>MSGSPAPQGALRQRIVASTPKKTKESKDGAASDAELDKLVKEAAAAKAPAGSERDYKIAFAIITALAFLTRFWGISHPDQVVFDEVHFGKFASYYLQRTYFFDVHPPLGKLLFAFMGWLVGYDGHFHFDNIGDPYVINKVPYVAFRALPAILGSLTVSVVFLIMWESGYSLPACILASGLVLLDNAHIGQTRLILLDATLVFAMACSLLCYIKFYKLRHEPFSRKWWKWLILTGFALSCDISTKYVGLFAFITIGSAVCIDLWDLLNINRPKGALTLPQFGKHFAARAFGLIFMPFMFYLFWFQVHFSILTRSGPGDDFMTPEFQETLSDNIMLANAVTIDYWDTITIKHKETKAYLHSHPDRYPLRYDDGRVSSQGQQVTGYPFNDTNNWWQILPAGPFEEPKLGRHVKHRDLVRLRHVGTDTYLLSHDVASPYYPTNQEFTTVSFNEAYGDRAADTLFEVRIEHGKPGQEFKSISSHFKLIHNPSKVAMWTHPTPLPDWGHRQQEINGNKQIAPSSNVWLVEDIVSLPADHKRREKPERKVKTLPFLRKWFELQRSMFWHNNQLTASHPYASLPYQWPFLLRGVSFWTNSETRQQIYFLGNPVGWWIASSVLAIYVGIVLADQFSLRRGIDALDHRTRSRLYNSTGFFFLAWATHYFPFFVMGRQLFLHHYLPAHLASTLVTGALVEFIFSPEAPEHEIAAQQAKSSSSGKRGGVAMKRHITARERFAGQSLMGSWIATAVILALVAWSWWFFLPLTYGYP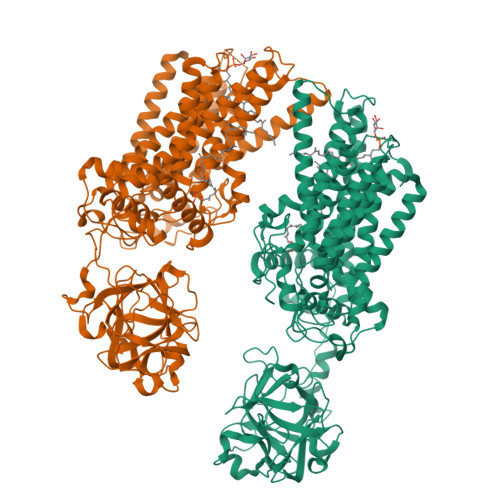GMSVQQVLRRKWLGYDLHFAKLEVLFQGPGSHHHHHHHHHH[2x]>[2x]MASDKFPVAENPSSSFKYESAVQYRPAPDSYLNPCPQAGRIVKETYTGINGTKSLNVYLPYGYDPNKKYNIFYLMHGGGENENTIFSNDVKLQNILDHAIMNGELEPLIVVTPTFNGGNCTAQNFYQEFRQNVIPFVESKYSTYAESTTPQGIAASRMHRGFGGFAMGGLTTWY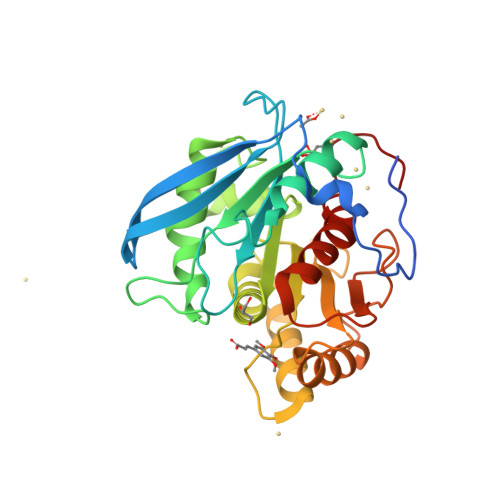VMVNCLDYVAYFMPLSGDYWYGNSPQDKANSIAEAINRSGLSKREYFVFAATGSEDIAYANMNPQIEAMKALPHFDYTSDFSKGNFYFLVAPGATHWWGYVRHYIYDALPYFFHELEHHHHHH> SVRDELRWVF;> VSYANAVSRAAPAVANLYTTKMVSKPSHPLFDDPMFRRFFGDNLPQQKRMESSLGSAVIMSAEGYLLTNNHVTAGADQIIVALRDGRETIAQLVGSDPETDLAVLKIDLKNLPAMTLGRSDGIRTGDVCLAIGNPFGVGQTVTMGIISATGRNQLGLNTYEDFIQTDAAINPGNAGGALVDAAGNLI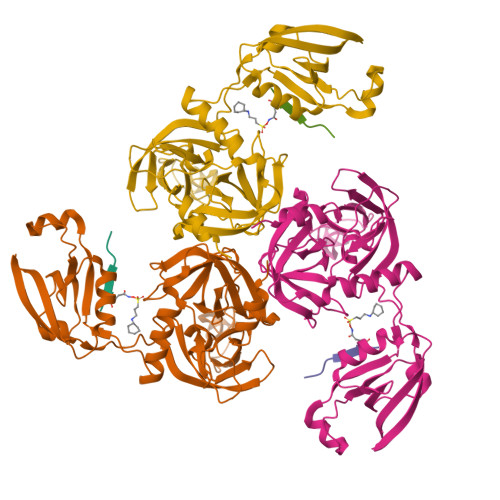GINTAIFSKSGGSQGIGFAIPTKLALEVMQSIIEHGQVIRGWLGVEVKALTPELAESLGLGETAGIVVAGVYRDGPAARGGLLPGDVILTIDKQEASDGRRSMNQVARTRPGQKISIVVLRNGQKVNLTAEVGLRPPPAPAP(2S)-2-[([1,1'-biphenyl]-4-yl)oxy]propanoic 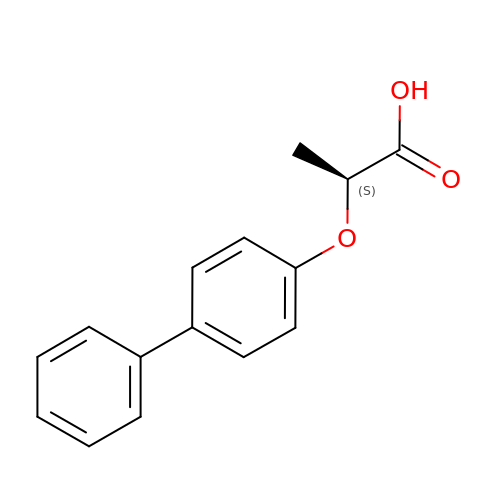acid | C15 H14 O3 | FUPGQEMJIGUBGO-NSHDSACASA-N> MAKTYLLEIGLEEMPAHVVTPSVLQLKERMIKFLKDARLDFEDVKTFSTPRRLTVQVLGLADKQADVKKEVRGPAKKIAQDADGNWTKAAIGFSKGQGASTDDIVFKDVKGTPYVFVQTFTAGKTAAEVLTGGIKDVITKMNFPTMMKWSTYSFKYIRPIRWIVSLLDDEVVPVQILDVAAGRVSRGHRFLGHDVEIATAADYEADLASVQVVADAAKRKATIREQIAALANERDWQIK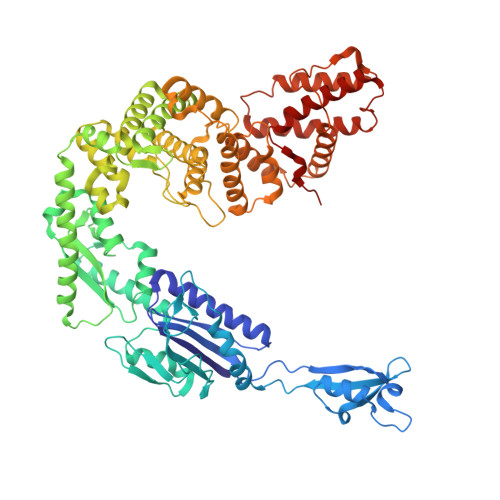VNEDLLEEVNNLVEYPTAFAGDFDTKYLTIPDEVLITSMRDHQRFFYVTDAEDNLLPHFVSVRNGNTDHLENVALGNQKVLTARLEDAAFFYHEDQQHSIQEYVERLKKVSFHDKIGTMYEKMQRVMIISDFLADRFGLTETEKNQLHRAAQIYKFDLVTGMVGEFPELQGVMGDKYAVLKGEDPAVGQAIREHYMPISADGDLPKSKVGAVLAIADKVDSITSFFAVGLTPSGSNDPFALRRQAFGIVRIVREQGWDFPIRQLEADIQKELVAHDATYNLDFEKQTAPVADFLTDRVKQWFNNRKIRYDIVDTVIKGSRQDIREMFKAADVLNAHQDDPQFKDTIEAFTRLLRITAKAKLAADDLTVDPSLFENEAEQHLYDAVLELQKQFTPAMSMEDRFKALAALRPLIVDYFEQTMVMSKDEKVRDNHLKQLLTIAQMINVMGDLNQLIVK> GSMAPITAYSQQTRGLLGCIITSLTGRDKNQVDGEVQVLSTATQSFLATCVNGVCWTVYHGAGSKTLAGPKGPITQMYTNVDQDLVGWPAPPGARSMTPCTCGSSDLYLVTRHADVIPVRRRGDSRGSLLSPRPVSYLKGSSGGPLLCPSGHVVGIFRAAVCTRGVAKAVDFIPVESMETTMRSPVF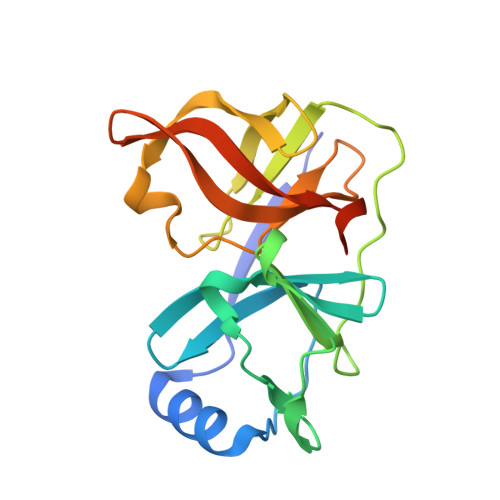TDN Adenylyl cyclase 9 (AC9) is a membrane-bound enzyme that converts ATP into cAMP. The enzyme is weakly activated by forskolin, fully activated by the G protein Gαs subunit and is autoinhibited by the AC9 C-terminus. Each membrane AC contains two conserved cytosolic catalytic domains and twelve predicted transmembrane (TM) helices, with cytosolic N- and C-termini of varied lengths and regulatory roles. Here, we present the cryo-EM structures of AC9 in several distinct states: (i) AC9 bound to a nucleotide inhibitor MANT-GTP, (ii) bound to an artificial activator (DARPin C4) and MANT-GTP, (iii) bound to DARPin C4 and a nucleotide analogue ATPαS, (iv) bound to Gαs and MANT-GTP.

To characterize the conformation of AC9 in the absence of G protein α subunit, we determined the structure of bovine AC9 in complex with MANT-GTP (an inhibitor we used to stabilize AC9), referred to as AC9–M throughout the text below, using cryo-EM and single-particle analysis at 4.9 Å resolution. Our choice of MANT-GTP as a ligand for the active site of AC9 was based on two considerations: (i) we have used it successfully in our previous studies of membrane ACs, (ii) the overall conformation of the AC catalytic domains stabilized by MANT-GTP is similar to that stabilized by ATP analogs, such as ATPαS, based on X-ray crystallographic studies. Due to the low molecular weight and innate flexibility and pseudo-two-fold symmetry of the full-length AC9, the resolution of the AC9–M reconstruction could not be improved beyond 4.9 Å. Although the cryo-EM maps of AC9–M and AC9–C4–M featured the density elements corresponding to a bound MANT-GTP molecule, the location of the nucleotide density in each of the maps was distinct from that observed in the previously determined AC91250–Gαs structure in the presence of MANT-GTP and forskolin (AC91250–Gαs–MF). The nucleotide density stretched out towards the forskolin binding site, suggesting that the molecule may have been captured in a previously undescribed orientation within the active site. The local resolution of this region in both density maps (AC9–M and AC9–C4–M) was not sufficiently high to unambiguously define the pose of MANT-GTP. Based on the available structures, the G protein-free state (nucleotide-bound state, corresponding to AC9–M) can transition to a partially active state upon Gαs binding (Gαs-bound state); subsequent binding of forskolin (Fsk) fully activates AC9 (Gαs/Fsk-bound state).

> MASPPHQQLLQHHSTEVSCDSSGDSNSVRVRINPKQPSSNSHPKHCKYSISSSCSSSGDSGGVPRRMGAGGRLRRRKKLPQLFERASSRWWDPKFDSVNLEEACMERCFPQTQRRFRYALFYIGFACLLWSIYFGVHMKSKLIVMVAPALCFLVVCVGFFLFTFTKLYARHYVWTSLVLTLLVFALTLAAQFQVLTPLSGRVDNFNHTRAARPTDTCLSQVGSFSMCIEVLFLLYTVMHLPLYLSLILGVAYSVLFETFGYHFQDEACFASPGAEALHWELLSRALLHLCIHAIGIHLFIMSQVRSRSTFLKVGQSIMHGKDLEVEKALKERMIHSVMPRIIADDLMKQGDEESENSVKRHATSSPKNRKKKSSIQKAPIAFRPFKMQQIEEVSILFADIVGFTKMSANKSAHALVGLLNDLFGRFDRLCEETKCEKISTLGDCYYCVAGCPEPRADHAYCCIEMGLGMIRAIEQFCQEKKEMVNMRVGVHTGTVLCGILGMRRFKFDVWSNDVNLANLMEQLGVAGKVHISEATAKYLDDRYEMEDGKVTERLGQSVVADQLKGLKTYLIAGQRAKESHCSCSEALLSGFEVLDGSRVSSGPRGQGTASPGSVSDLAQTVKTFDNLKTCPSCGITFTPKPEAGAEGGAVQNGCQEEPKNSAKASGGPSSKTQNGLLSPPPEEKLTNSQTSLCEILQEKGRWAGVSLDQSALLPLRFKNIREKTDAHFVDVIKEDSLMKDYFFKPPINQFSLNFLDPELERAYRTSYQEEVVKSSPVRTFASATFSSLLDVLLSTTVFLILSITCFLRYGAASTPPPPAALAVFGAALLLEILSLVVSVRMVFFLEDVMTCTKRLLEWIAGWLPRHFIGAILVSLPALAVYSHVTSEFETNIHSTMFTGSAVLTAVVQYCNFCQLSSWMRSSLATVVGAGPLLLLLYVSLCPDSSTVISHLDAVQNFSSTRKLCNASLPHDGRSPASLIGQEVILVFFLLLLLVWFLNREFEVSYRLHYHGDVEADLHRTKIQSMRDQADWLLRNIIPYHVAEQLKVSQTYSKNHDSGGVIFASIVNFSEFYEENYEGGKECYRVLNELIGDFDELLSKPDYSSIEKIKTIGATYMAASGLNATQCRDGSHPQEHLQILFEFAKEMMRVVDDFNNNMLWFNFKLRVGFNHGPLTAGVIGTTKLLYDIWGDTVNIASRMDTTGVECRIQVSEESYRVLSKMGYEFDYRGTVNVKGKGQMKTYLYPKCTDSGLVPQHQLSISPDIRVQVDGSIGRSPTDEIASLVPSVQNPDQVPPGSENNAQTRDAHPSAKRPWKEPVRAEERCRFGKAIEKSDCEEVGMEEANELTKLNVSERA> EYEVELKKTGQIFTVSPGSTLLQACLDNDVRIEASCEQGVCGTCITPVVSGDLEHHDTYLSKKERESGKWIMPC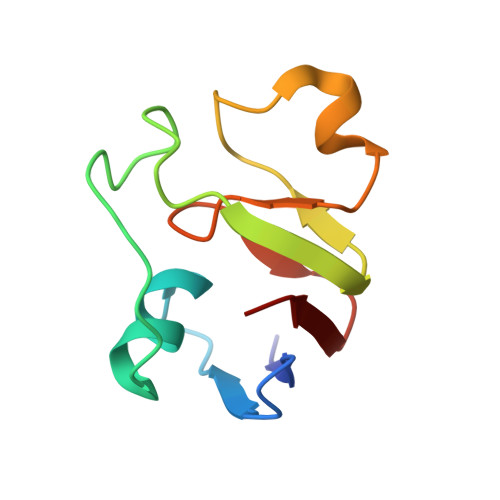VSRCKSKKIVLDL>[3x]GPAMLPISMSDEGDSFLVKDSLGENKIPKNPSKVVILDLGILDTFDALKLNDKVVGVPAKNLPKYLQQFKNKPSVGGVQQVDFEAINALKPDLIIISGRQSKFYDKLKEIAPTLFVGLDNANFLSSFENNVLSVAKLYGLEKEALEKISDIKNEIEKAKSIVDEDKKALIILTNSNKISAFGPQSRFGIIHDVLGINAVDENIKVGTLGKSINSEFILEKNPDYIFVVDRNVILGNKERAQGILDNALVAKTKAAQNKKIIYLDPEYWYLASGNGLESLKTMILEIKNAVK

The periplasmic binding protein (PBP) CeuE1 is an important component of the Fe(III) uptake system in Campylobacter jejuni, a commensal Gram-negative bacterium in the avian gut, but a common source of food poisoning in humans. CeuE, an integral part of the CeuBCDE ABC transporter of C. jejuni, is responsible for capturing Fe(III)-siderophore complexes in the periplasm for delivery to their respective inner membrane transporter. C. jejuni does not itself synthesize siderophores, but capitalizes on their secretion by other bacteria, such as E. coli. Here we report a combined solution and structural study of a series of synthetic tetradentate analogues of the enterobactin-derived bis(2, 3-dihydroxybenzoyl-L-Ser), to explore the ligand-binding promiscuity of CeuE, both wild type and with mutations of the Fe(III) binding residues H227 and Y288.

To probe the relative contributions of His227 and Tyr288 to Fe(III)-siderophore binding, site-directed mutagenesis was then used to replace the side chains of the two Fe(III)-coordinating amino acids with non-coordinating side chains of similar size. His227 was mutated to either leucine (H227L) or alanine (H227A), while Y288 was mutated to phenylalanine (Y288F). All five mutants (Y288F, H227L, H227A, H227L/Y288F, H227A/Y288F) were crystallized in their apo form, and all structures are closely similar to that of wild type CeuE. However while there is clear electron density for the Y288F mutation in its three structures, H227L and H227A are located in a flexible loop region and there is generally no electron density to confirm their presence. Mutants H227L and H227A gave Kd values of 22 ± 10 nM and 35 ± 14 nM, respectively, indicating only slightly weaker binding than for wild type, which indicates that the tyrosinate O-donor binds the Fe(III) cation more strongly than the histidine N-donor. The Λ-configuration signal was observed for mutants H227L and H227A, indicating that these do indeed bind Λ-Fe-5-Lic. The Λ-configuration was observed for all four, but with a decrease in signal amplitude compared to wild type, confirming the reduced binding affinity observed in the fluorescence quenching experiments.> SSPADSYNEGVKLQPQEISPPPTANLDRSNDKVYENVTGLVKAVIEMSSKIQPAPP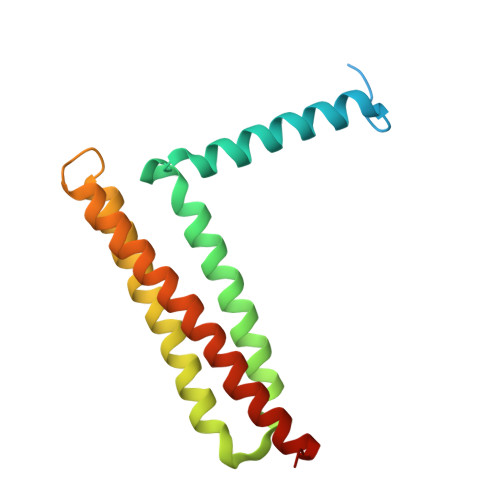EEYVPMVKEVGLALRTLLATVDETIPLLPASTHREIEMAQKLLNSDLGELINKMKLAQQYVMTSLQQEYKKQMLTAAHALAVDAKNLLDVIDQARLKMLGQTRPH>[2x]TELTKCKVSHAIKDIDGYQGISLLEWACVLFHTSGYDTQAVVNDNGSTEYGLFQISDRFWCKSSEFPESENICGISCDKLLDDELDDDIACAKKILAIKGIDYWKAYKPMCSEKLEQWRCEKP;>[2x]ASMTGGQ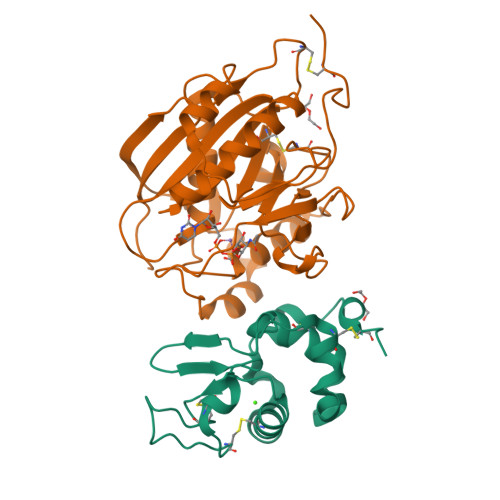QMGRGSSLTACPEESPLLVGPMLIEFNIPVDLKLVEQQNPKVKLGGRYTPMDCISPHKVAIIIPFRNRQEHLKYWLYYLHPILQRQQLDYGIYVINQAGESMFNRAKLLNVGFKEALKDYDYNCFVFSDVDLIPMNDHNTYRCFSQPRHISVAMDKFGFSLPYVQYFGGVSALSKQQFLSINGFPNNYWGWGGEDDDIYNRLAFRGMSVSRPNAVIGKCRMIRHSRDKKNEPNPQRFDRIAHTKETMLSDGLNSLTYMVLEVQRYPLYTKITVDIGTPS>MKGLAMLGIGRIGWIEKKIPECGPLDALVRPLALAPCTSDTHTVWAG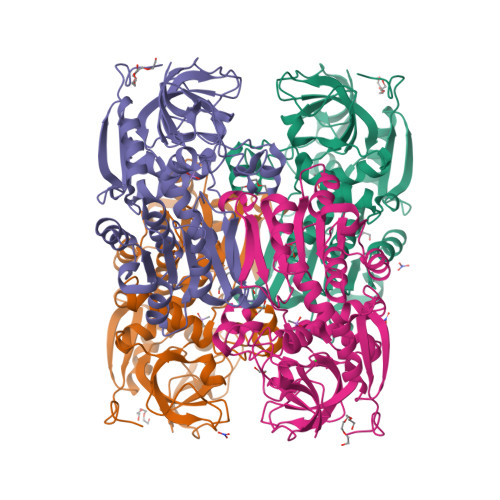AIGDRHDMILGHEAVGQIVKVGSLVKRLKVGDKVIVPAITPDWGEEESQRGYPMHSGGMLGGWKFSNFKDGVFSEVFHVNEADANLALLPRDIKPEDAVMLSDMVTTGFHGAELANIKLGDTVCVIGIGPVGLMSVAGANHLGAGRIFAVGSRKHCCDIALEYGATDIINYKNGDIVEQILKATDGKGVDKVVIAGGDVHTFAQAVKMIKPGSDIGNVNYLGEGDNIPIPRSEWGVGMGHKHIHGGLTPGGRVRMEKLASLISTGKLDTSKLITHRFEGLEKVEDALMLMKNKPADLIKPVVRIHYDDEDTLH[4x]> HMQLEIQVALNFIISYLYNKLPRRRVNIFGEELERLL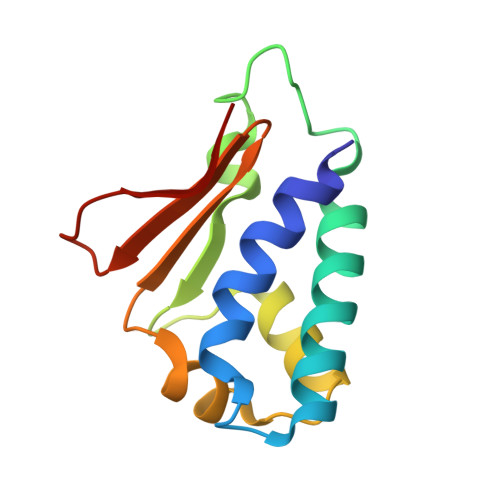KKKYEGHWYPEKPYKGSGFRCIHIGEKVDPVIEQASKESGLDIDDVRGNLPQDLSVWIDPFEVSYQIGEKGPVKVLYVD> MAESTTLETIEIHPITFPPEVLARISPELSLQRHLSLGIRPCLRKYEEFRDVAIENNTLSRYADAGNIDTKNNILGSNVLKSGKTIVITSITGGIIEETSAAIKDLDDFGEEELFEVTKEEDIIANYASVYPVVEVERGRVGACTDEEMTISQKLHDSILHSRILPKKALKVKAGVRSANEDGTFSVLYPDELEDDTLNETNLKMKRKWSYVLYAKIVVLSRTGPVFDLCWNSLMYALQSVKLPRAFIDERASDLRMTIRTRGRSATIRETYEIICD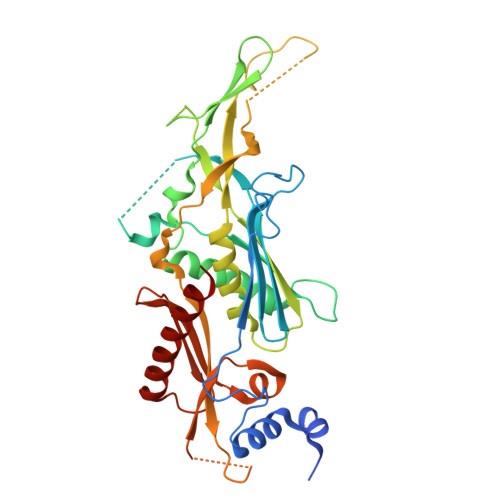QTKSVPLMINAKNIAFASNYGIVELDPECQLQNSDNSEEEEVDIDMDKLNTVLIADLDTEAEETSIHSTISILAAPSGNYKQLTLMGGGAKITPEMIKRSLLLSRVRADDLSTRFNI>NISYTEGAKPGAISAPVAISRRVAGMKPRFVRSEGSVKIVHREFIASVLPSNDLTVNNGDVNIGKYRVNPSNNALFTWLQGQAQLYDMYRFTRLRFTYIPTTGSTSTGRVSILWDRDSQDPLPIDRAAISSYAHYADSAPWAENVLVVPCDNTWRYMNDTNAVDRKLVDFGQFLFATYSGAGATAHGDLYVEYAVEFKDPQPIAGMVCMFDRLVSFSEVGSTIKGVNYIADRDVITTGGNIGVNINIPGTYLVTIVLNATSIGSLTFTGNSKLVGNSLNVTSSGASALTFTLNSTGVPNSSNSSFSVG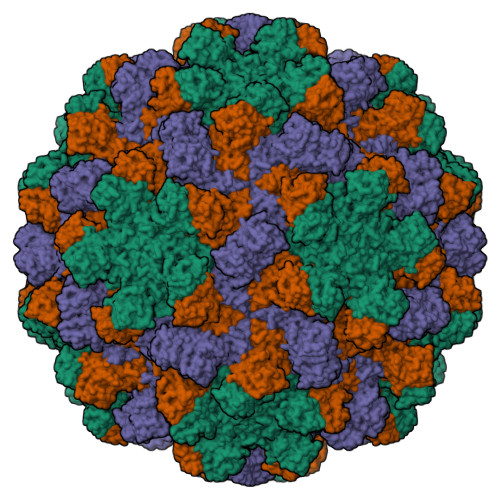TVVALTRVRMTITRCSPETAYLA[3x]Stimulated by the first neuraminidase (NA) crystal structures, the NAIs were designed to interact with the active site of all NA types. We identified a novel isoleucine to arginine change at position 223 (I223R) in the NA of a virus isolated from an immune suppressed child on prolonged oseltamivir and zanamivir therapy. In contrast to the frequently observed H275Y change, which causes selective resistance to oseltamivir, the I223R mutation conferred a resistance phenotype against both oseltamivir and zanamivir. Our results support this suggestion by indicating that a ligand-free form of the pandemic neuraminidase adopts an open conformation. Together with this structure we present the structures of the I223R mutant neuraminidase in complex with oseltamivir and zanamivir to investigate the resistance mechanism of the I223R mutant neuraminidase.

Crystals of wild type and mutant neuraminidases were grown in the absence or presence of the oseltamivir and zanamivir neuraminidase inhibitors. In the wild type N1 neuraminidase structure, a small pocket, the “223-pocket”, also adjacent to the active site, but distinct from the 150-cavity, contains two water molecules.

>[4x]VKLAGNSSLCPVSGWAIYSKDNSVRIGSKGDVFVIREPFISCSPLECRTFFLTQGALLNDKHSNGTIKDRSPYRTLMSCPIGEVPSPYNSRFESVAWSASACHDGINWLTIGISGPDNGAVAVLKYNGIITDTIKSWRNNILRTQESECACVNGSCFTVMTDGPSNGQASYKIFRIEKGKIVKSVEMNAPNYHYEECSCYPDSSEITCVCRDNWHGSNRPWVSFNQNLEYQIGYICSGIFGDNPRPNDKTGSCGPVSSNGANGVKGFSFKYGNGVWIGRTKSISSRNGFEMIWDPNGWTGTDNNFSIKQDIVGINEWSGYSGSFVQHPELTGLDCIRPCFWVELIRGRPKENTIWTSGSSISFCGVNSDTVGWSWPDGAELPFTIDK> MYDWFKQMRKESPVYYDGKVWNLFKYEDCKMVLNDHKRFSSNLTGYNDKLEMLRSGKVFFDIPTRYTMLTSDPPLHDELRNLTADAFNPSNLPV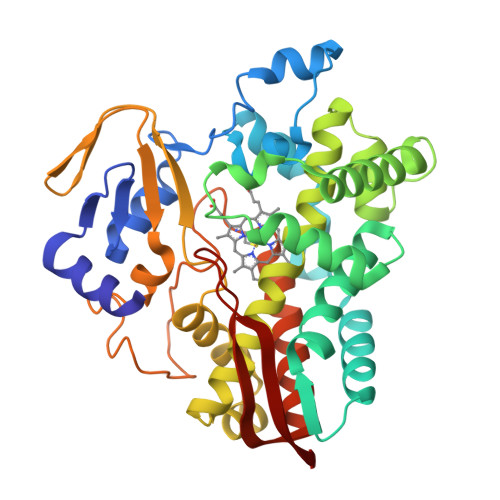DFVREVTVKLLSELDEEFDVIESFAIPLPILVISKMLGINPDVKKVKDWSDLVALRLGRADEIFSIGRKYLELISFSKKELDSRKGKEIVDLTGKIANSNLSELEKEGYFILLMIAGNETTTNLIGNAIEDFTLYNSWDYVREKGALKAVEEALRFSPPVMRTIRVTKEKVKIRDQVIDEGELVRVWIASANRDEEVFKDPDSFIPDRTPNPHLSFGSGIHLCLGAPLARLEARIALEEFAKKFRVKEIVKKEKIDNEVLNGYRKLVVRVERT> MKKYTCTVCGYIYNPEDGDPDNGVNPGTDFKDIPDDWVCPLCGLG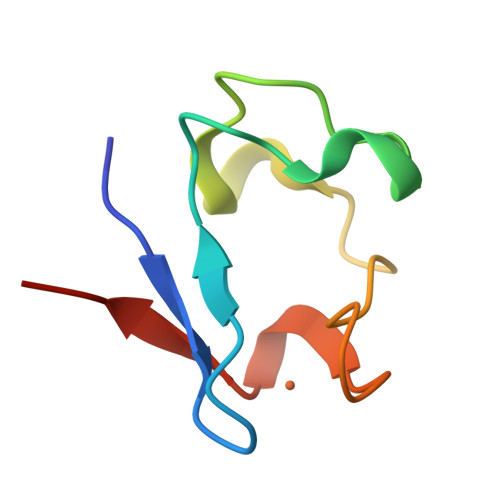KDQFEEVEE> MPTAGSELPRRPLPPAAQER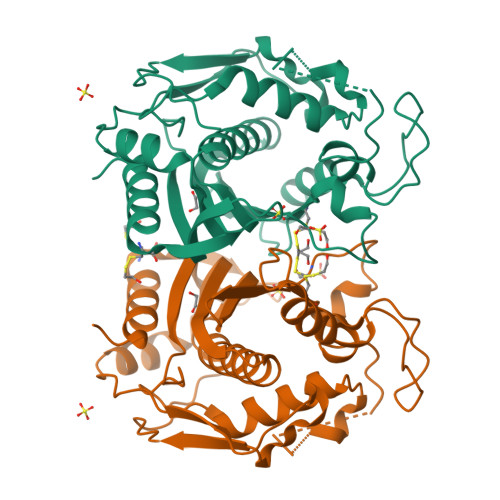DAEPRPPHGELQYLGQIQHILRCGVRKDDRTGTGTLSVFGMQARYSLRDEFPLLTTKRVFWKGVLEELLWFIKGSTNAKELSSKGVKIWDANGSRDFLDSLGFSTREEGDLGPVYGFQWRHFGAEYRDMESDYSGQGVDQLQRVIDTIKTNPDDRRIIMCAWNPRDLPLMALPPCHALCQFYVVNSELSCQLYQRSGDMGLGVPFNIASYALLTYMIAHITGLKPGDFIHTLGDAHIYLNHIEPLKIQLQREPRPFPKLRILRKVEKIDDFKAEDFQIEGYNPHPTIKMEMAV>MFTEIMRYVLDLGPTVMLPIVVILFSLLLKMKPGDAFKSGIHIGIGFVGIGLVIGLMLDSIGPAAKAMAEAFDINLKVVDIGWPGSSPMTWASQIALIAIPIAIVVNLVMLMTRMTRVVNVDIWNIWHMTFTGALVHIATGSYALAIVGVVVHAAFVYKLGDWFAKDTRDFFGLDGIAIPHGTSAYLGPIAVLVDTVIEKIPGLNRIHFSADDVQKRFGAFGEPVTIGFVMGLVIGLLAGYEIKAVLQLAVKTAAVMLLMPRVIKPIMDGLTPIAKQARSRLQAKFGGQDFLIGLDPALLLGHTSVVSASLIFIPLTILIAVVTPGNQVLPFGDLATIGFFVAMAVA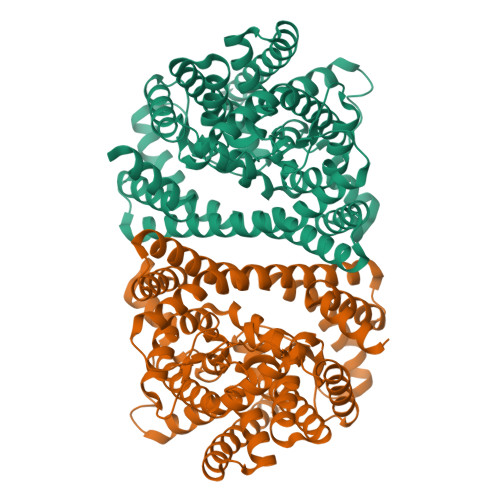VHQGNLFRTLISGVIIMSITLWIATQTIGLHTQLAANAGSLTGDGSLVASMDQGGSPITYLLVQALTLENVIGLVAIGALYGIGIFLTWRRAKRFAAQAESPANVQVQAAGQSLESSGENLYFQ[2x]> GGUUGCCGAAUCCCCUAGAAAGGUACGGAGGAACCGCUUUUUGGGGUUAAUCUGCAGUGAAGCUGCAGU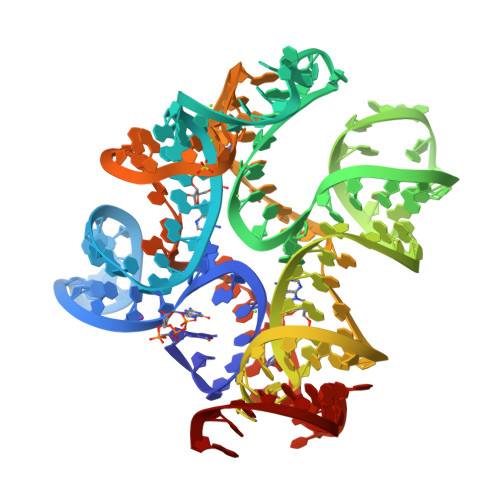AGGGAUACCUUCUGUCCCGCACCCGACAGCUAACUCCGGAGGCAAUAAAGGAAGGAG>[2x]MSIKIRDFGLGSDLISLTNKAGVTISFTNLGARIVDWQKDGKHLILGFDSAKEYLEKDAYPGATVGPTAGRIKDGLVKISGKDYILNQNEGPQTLHGGEESIHTKLWTYEVTDLGAEVQVKFSLVSNDGTNGYPGKIEMSVTHS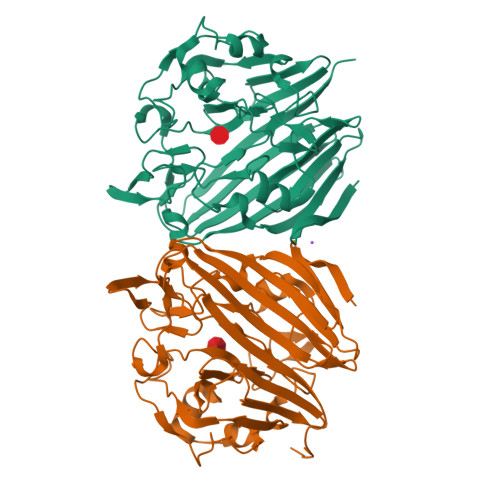FDDDNKWKIHYEAISDKDTVFNPTGHVYFNLNGDASESVENHGLRLAASRFVPLKDQTEIVRGDIVDIKNTDLDFRQEKQLSNAFNSNMEQVQLVKGIDHPFLLDQLGLDKEQARLTLDDTSISVFTDQPSIVIFTANFGDLGTLYHEKKQVHHGGITFECQVSPGSEQIPELGDISLKAGEKYQATTIYSLHTKLEHHHHHH N-(2,1,3-Benzothiadiazol-5-yl)acetamide | C8 H7 N3 O S | 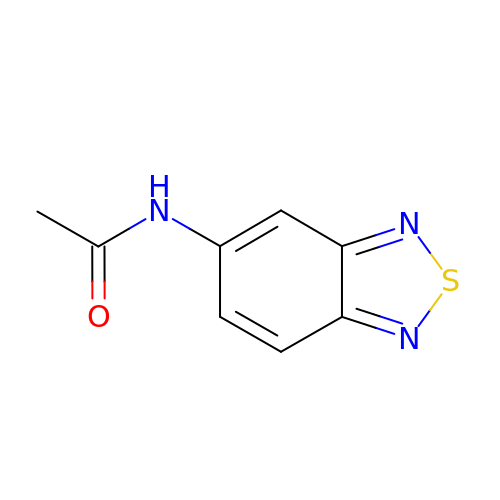DCJCIZAANYCYFG-UHFFFAOYSA-N> AYACSFPPSEIPGSKECLAEALQKHQGFKKKSYALICAYLNYKEDAENYERAAEDFDSAVKCTG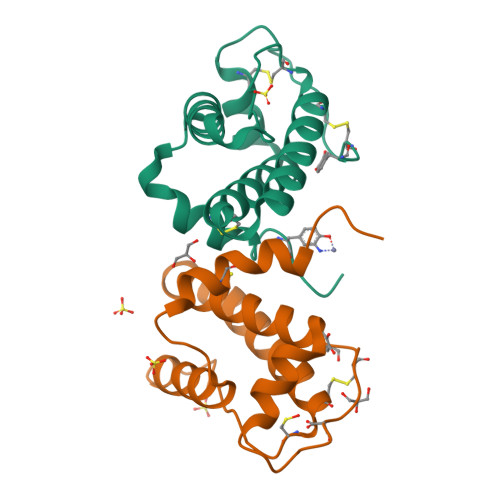CKEGVDLHEGNPELIEEGFEKFLASLKIDRKALGSLCTLFQKLYAIPHN;> AYACSFPPGEIPGSKECLAEALQKHQGFKKKSYALICAYLNYKEDAENYERAAEDFDSAVKCTGCKEGVDLHEGNPELIEEGFEKFLASLKIDRKALGSLCTLFQKLYAIPHN>MHHHHHHLVPRGSEDELYRQSLEIISRYLREQATGAKDTKPMGRSGATSRKALETLRRVGDGVQRNHETAFQGMLRKLDIKNEDDVKSLSRVMIHVFSDGVTNWGRIVTLISFGAFVAKHLKTINQESCIEPLAESITDVLVRTKRDWLVKQRGW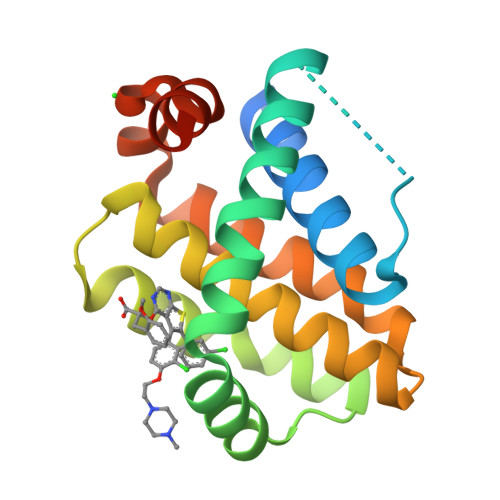DGFVEFFHVEDLEGG[2x]> QQKPVVKTAQNLAEVNGPETLIGPGAKEGTVPTDLDQETGLARLELLGKLEGIDVFDTKPLDS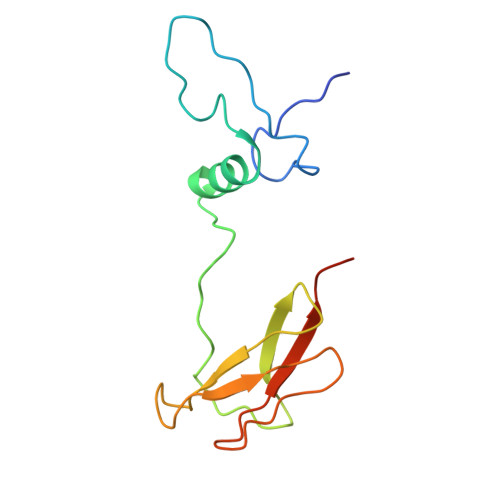SRKGTMKDPIIIESYDDYRYVGCTGSPAGSHTIMWLKPTVNEVARCWECGSVYKLNPVGVPNDDHHH> TQAKAKHADVPVNLYRPNAPFIGKVISNEPLVKEGGIGIVQHIKFDLTGGNLKYIEGQSIGIIPPGVDKNGKPEKLRLYSIASTRHGDDVDDKTISLCVRQLEYKHPESGETVYGVCSTYLTHIEPGSEVKITGPVGKEMLLPDDPEANVIMLATGTGIAPMRTYLWRMFKDAERAANPEYQFKGFSWLVFGV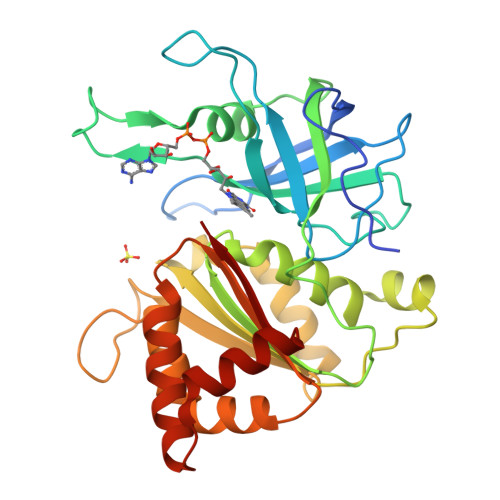PTTPNILYKEELEEIQQKYPDNFRLTYAISREQKNPQGGRMYIQDRVAEHADQLWQLIKNQKTHTYICGPRGMEEGIDAALSAAAAKEGVTWSDYQKDLKKAGRWHVETY> GLPVLNTPGSNQYLTSDNHQSPCAIPEFDVTPPIDIPGEVKNMMELAEIDTMIPLNLESTKRNTMDMYRVTLSDSADLSQPILCLSLSPAFDPRLSHTMLGEVLNYYTHWAGSLKFTFLFCGSMMATGKILVAYAPPGAQPPTSRKEAMLGTHVIWDLGLQSSCTMVVPWISNVTYRQTTQDSFTEGGYISMFY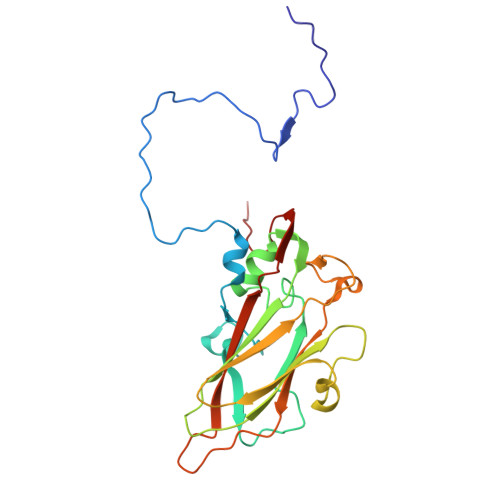QTRIVVPLSTPKSMSMLGFVSACNDFSVRLLRDTTHISQSA>GPDRSFRWKYHQFRFLCHSNALPSHVKISVSRQTLFEDSFQQIMNMKPYDLRRRLYIIMRGEEGLDYGGIAREWFFLLSHEVLNPMYCLFEYAGKNNYCLQINPASSINPDHLTYFRFIGRFIAMALYHGKFIDTGFTLPFYKRMLNKRPTLKDLESIDPEFYNSIVWIKENNLEECGLELYFIQDMEILGKVTTHELKEGGESIRVTEENKEEYIMLLTDWRFTRGVEEQTKAFLDGFNEVAPLEWLRYFDEKELELMLCGMQEIDMSDWQKSTIYRHYTKNSKQIQWFWQVVKEMDNEKRIRLLQFVTGTCRLPVGGFAELIGSNGPQKFCIDKVGKETWLPRSHTCFNRLDLPPYKSYEQLREKLLYAIEETE[2x];> XDPAQMYCREAAFYCFMHX

Here, we report a general and rapid method for discovering α-helically constrained (Helicon) polypeptides that cooperatively induce the interaction between two target proteins without relying on previously known binders or an intrinsic affinity between the proteins. We show that Helicons are capable of binding every major class of E3 ubiquitin ligases, which are of great biological and therapeutic interest but remain largely intractable to targeting by small molecules. In addition to possessing increased stability and membrane permeability, Helicons are capable of binding large, flat protein surfaces that are inaccessible to targeting by small molecules, and Helicons have been developed to target a range of PPI targets in cells and in vivo. Characterizing Helicon-E3 co-structures and mechanisms of action, we identified new binding sites for α-helices on the E3 surfaces, as well as potential probes of the disease-linked E3, WWP123,24, highlighting the generality of our approach against this therapeutically important target class.

First, we focused on the NEDD4-like E3 ligases, which make up approximately a third of the HECT family. These include WWP1 and WWP2, which each consist of four tandem WW domains and a catalytic HECT domain at the C-terminus that transfers ubiquitin from a bound E2 first to itself and subsequently to the target substrate. We next solved the crystal structures of five Helicons, four in complex with WWP2HECT representing all three groups of HECT-binding clusters, and one from Group 1 with WWP1HECT. These structures revealed three distinct Helicon binding sites on WWP2HECT. In all of the structures, we found that the HECT domains adopted similarly closed (inhibited) conformations. We found that individual Helicons from all three HECT-binding Groups (1–3) could modestly inhibit the auto-ubiquitylation activity of the isolated WWP2HECT.SadB is a trimeric lipoprotein located in the inner membrane of Salmonella spp., with homologs in other enterobacteria, including pathogenic E. coli species. The sadB gene is located in an operon with sadA; orthologous operons are only found in enterobacteria, whereas other TAAs are not typically associated with lipoproteins. In this study, we determined the three-dimensional structure of SadB using x-ray crystallography and show that SadB enhances the surface display of SadA, suggesting a direct involvement of SadB in the autotransport mechanism of the trimeric autotransporter adhesin SadA. The reduced amount and increased stickiness of surface-localized SadA in the absence of SadB and the decreased resistance of SadA to proteinase K in the absence of SadB all suggest a direct influence of SadB on SadA export and folding.

To obtain the structure of SadB, a construct lacking the N-terminal signal peptide and replacing the lipid-modifiable cysteine residue Cys-22 by a serine residue was created. The resulting protein was solubly expressed in the cytosol without the lipid anchor. Crystallization trials yielded crystals diffracting to 2.45 Å. After initial attempts to solve the structure via molecular replacement with the NMR structure of YajI (2JWY) were not fruitful, we were able to solve it via single isomorphous replacement using a platinum derivative. Like SadA, SadB is a homotrimer; it is held together by an extended N-terminal coiled coil of nine heptads, which leads into three separate globular C-terminal domains of β-sandwich topology, each composed of two antiparallel β-sheets. In this variant of the Ig fold, the first sheet has the strand order β-1, β-8, β-5, and β-6, whereas the loop connecting β-5 and β-6 is especially long and includes a short α-helix protruding toward the N terminus. The second sheet has strand order β-2, β-3, β-4, and β-7. In tracing the electron density of this domain, the YajI structure was very helpful as it has the identical topology. Trimerization of the protein was not observed during protein purification, including size exclusion chromatography, suggesting a low trimerization propensity of the coiled coil. We ascribe this to the high number of polar residues in core positions of the coiled-coil domain.

>[3x]MSDYFADKHLVEEMKEQQKEQETKINLLEKQQKEQEAKINLLEKQQATIINTTKKVTEVVGRVERKQRLFDYTELDPSQTHYFIINNGNIGLAGRILSIEPIDNGSVIHLDLVNLLSIPVSNLAFNMTWGTKKPSEAKDLPRWKQLLLNTKMDSTIELLPGAWTNVTLTLKGVSPNNLKYLKIGIDMENVIFDSIQPINDTKKKPKK>SNAMKKVAVLLAPGFEEAEAIVTLDILRRLHIDVETLACAESRAVVSYHDIPMVADSTLSERQQALFDAVVLPGGPQGSANLAANPAVIAFVARHDAAGKLICPIASAAARVLGAHGLLKGRRYVCSGDLWKAVPEGVYVDAPVV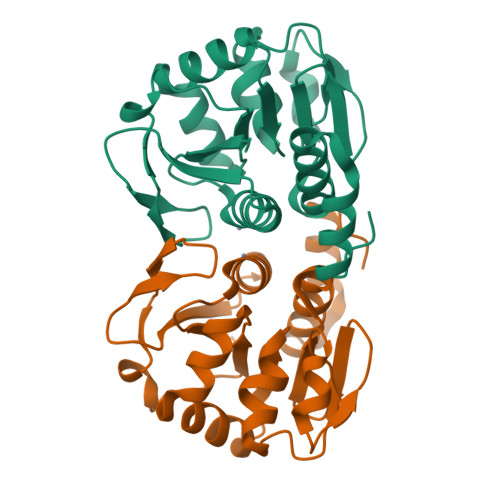EDGNLISGKGLGHVFDFALTLSARLLGDDAPVREQAEHIYYPW[14x]> MLRALWLFWILVAITVLFSKRCSAQESLSCDASGVCDGRSRSFTSIPSGLTAAMKSLDLSFNKITYIGHGDLRACANLQVLILKSSRINTIEGDAFYSLGSLEHLDLSDNHLSSLSSSWFGPLSSLKYLNLMGNPYQTLGVTS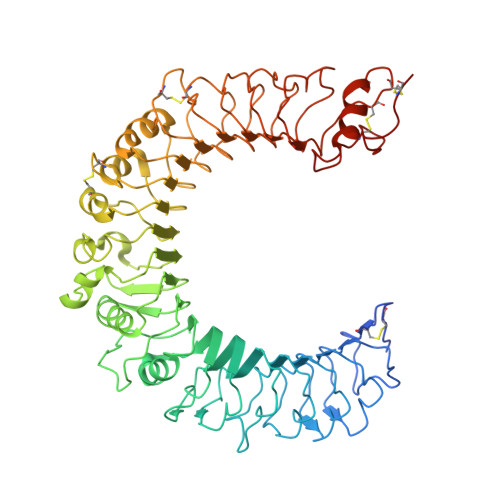LFPNLTNLQTLRIGNVETFSEIRRIDFAGLTSLNELEIKALSLRNYQSQSLKSIRDIHHLTLHLSESAFLLEIFADILSSVRYLELRDTNLARFQFSPLPVDEVSSPMKKLAFRGSVLTDESFNELLKLLRYILELSEVEFDDCTLNGLGDFNPSESDVVSELGKVETVTIRRLHIPQFYLFYDLSTVYSLLEKVKRITVENSKVFLVPCSFSQHLKSLEFLDLSENLMVEEYLKNSACKGAWPSLQTLVLSQNHLRSMQKTGEILLTLKNLTSLDISRNTFHPMPDSCQWPEKMRFLNLSSTGIRVVKTCIPQTLEVLDVSNNNLDSFSLFLPRLQELYISRNKLKTLPDASLFPVLLVMKIASNQLKSVPDGIFDRLTSLQKIWLHTNPWDCSCPRIDYLSRWLNKNSQKEQGSAKCSGSGKPVRSIICPTLVPR> GPLGSPE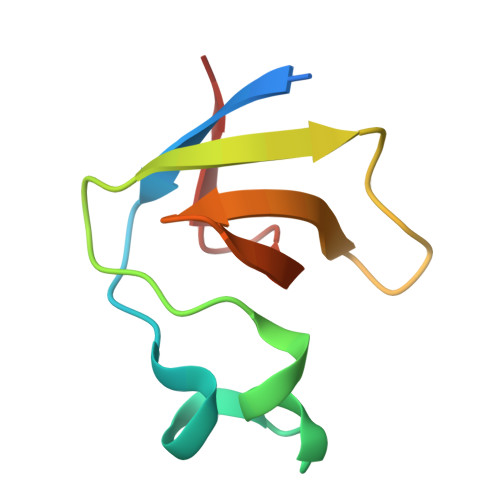FRYFVAMFDYDPSTMSPNPDGCDEELPFQEGDTIKVFGDKDADGFYWGELRGRRGYVPHNMVSEVE>MGGHHHHHHGENLYFQGISSETGEMGILWEFDPIINKWIRLSMKLKVERKPFAEGALREAYHTVSLGVGTDENYPLGTTTKLFPPIEMISPISKNNEAMTQLKNGTKFVLKLYKKEAEQQASRELYFEDVKMQMVCRDWGNKFNQKKPPKKIEFLMSWVVELIDRSPSSNGQPILCSIEPLLVGEFKKNNSNYGAVLTNRSTPQAFSHFTYELSNKQMIVVDIQGVDDLYTDPQIHTPDGKGFGLGNLGKAGINKFITTHKCNAVCALLDLDVKLGGVLSGNNKKQLQQGTMVMPDILPELMPSDNT[2x]

Dictyostelium myosin-II heavy chain kinase A (MHCK-A) phosphorylates the α-helical coiled-coil tail of myosin-II, causing contractile bipolar filaments of myosin-II to disassemble into inactive monomers. MHCK-A is a member of the atypical α-kinase family of serine/threonine protein kinases. The α-kinase domain is bi-lobed, with the active site located in a large cleft at the junction of the two lobes. The α-kinase N-lobe is similar to the N-lobe of other protein kinases but the C-lobe has a distinctive structure and requires a tightly bound zinc atom for stability.

Adenine binds into the far left-hand portion of the catalytic cleft, with the ribose moiety and phosphoryl groups extending towards the middle of the cleft. In all nucleotide-bound structures of A-CAT the left-hand side of the catalytic cleft is in a closed conformation with the P-loop clamped down over the adenine base, ribose moiety and phosphoryl groups. Hydrophobic interactions with the adenine base are made by Phe586 in the β5 strand and Val643 in the β7 strand. These two residues form part of a hydrophobic catalytic spine, comparable to that described in conventional protein kinases, that connects the N-lobe through the adenine base to the αD helix in the C-lobe. The invariant Lys645 residue in the β7 strand is also involved in binding the nucleotide through formation of a hydrogen bond with the adenine N2 atom.>MQREKVDVLVIGAGPAGTVAASLVNKSGFKVKIVEKQKFPRFVIGESLLPRCMEHLDEAGFLDAVKAQGFQQKFGAKFVRGKEIADFNFSDQFSNGWNWTWQVPRGNFDKTLADEAARQGVDVEYEVGVTDIKFFGTDSVTTIEDINGNKREIEARFIIDASGYGRVIPRMFGLDKPSGFESRRTLFTHIKDVKRPVAAEMEGNRITAVVHKPKVWIWVIPFSNGNTSVGFVGEPSYFDEYTGTPEERMRAMIANEGHIAERFKSEEFLFEPRTIEGYAISASKLYGDGFVLTGNATEFLDPIFSSGATFAMESGSKGGKLAVQFLKGEEVNWEKDFVEHMMQGIDTFRSFVTGWYDGTLHAVFFAKNPDPDHKRMICSVLAGYVWDKNNPFVKKHNTILKTLAKVIQMGEEALEH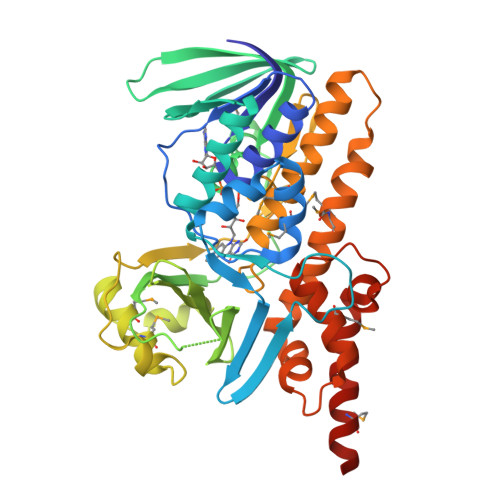HHHHH[8x]>[2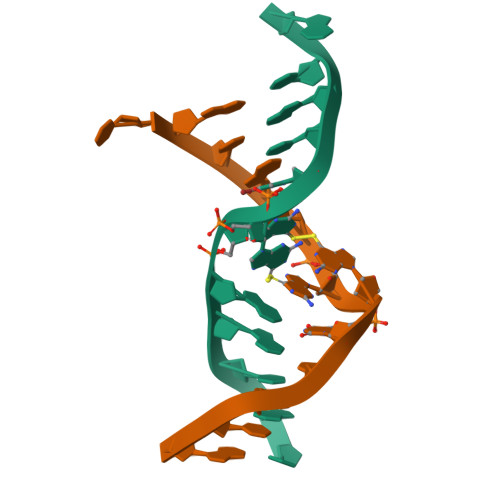x]CGCGAGGUCGCG> MDTEVYESPYADPEEIRPKEVYLDRKLLTLEDKELGSGNFGTVKKGYYQMKKVVKTVAVKILKNEANDPALKDELLAEANVMQQLDNPYIVRMIGICEAESWMLVMEMAELGPLNKYLQQNRHVKDKNIIELVHQVSMGMKYLEESNFVHRDLA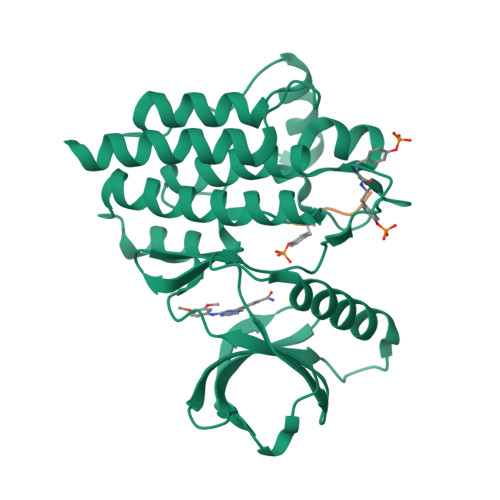ARNVLLVTQHYAKISDFGLSKALRADENYYKAQTHGKWPVKWYAPECINYYKFSSKSDVWSFGVLMWEAFSYGQKPYRGMKGSEVTAMLEKGERMGCPAGCPREMYDLMNLCWTYDVENRPGFAAVELRLRNYYYDVVNHHHHHH;> EVYESP>[6x]SVRDELRWVF;>MPKALRFLGWPVLVGVLLALLIIQHNPELVGLPRQEVHVEQAPLLSRLQEGPVSYANAVSRAAPAVANLYTTKMVSKPSHPLFDDPMFRRFFGDNLPQQKRMESSLGSAVIMSAEGYLLTNNHVTAGADQIIVALRDGRETIAQLVGSDPETDLAVLKIDLKNLPAMTLGRSDGIRTGDVCLAIGNPFGVGQTVTMGIISATGRNQLGLNTYEDFIQTDAAINPGNSGGALVDAAGNLIGINTAIFSKSGGSQGIGFAIPTKLALEVMQSIIEHGQVIRGWLGVEVKALTPELAESLGLGETAGIVVAGVYRDGPAARGGLLPGDVILTIDKQEASDGRRSMNQVARTRPGQKISIVVLRNGQKVNLTAEVGLRPPP[6x]

AlgW, a membrane-bound periplasmic serine protease belonging to the HtrA protein family, is a key regulator of the regulated intramembrane proteolysis (RIP) pathway and is responsible for transmitting the envelope stress signals in Pseudomonas aeruginosa. The AlgW PDZ domain senses and binds the C-terminal of mis-localized outer membrane proteins (OMPs) or periplasmic protein MucE, leading to catalytic activation of the protease domain. HtrA protease is characterized by its trypsin-like catalytic domain and regulatory PDZ domain; the catalytic triad was surrounded by several loops (L1, L2, L3, LD, LA) but, usually, in an inactive mode, and could be activated by sensing a specific molecular stimulus. The catalytic triad (H123, D153, and S227) sites are located between two β-barrels and are surrounded by activation loops L1 to L3, LD, and LA (named according to DegS nomenclature).

Protein samples were mixed with two types of peptide activator (tripeptide WVF, decapeptide SVRDELRWVF) prior to crystallization trials, yielding four complex structures, AlgW-tripeptide, AlgWS227A-tripeptide, AlgW-decapeptide, and AlgWS227A-decapeptide, with resolutions from 1.8 to 2.6 Å. In AlgW-decapeptide, each asymmetric unit contains a DegP-like hexamer that is stacked by two interlocked basic trimers arranged in a face-to-face manner, whereas the intertrimer contacts are stabilized by the long LA loop extending from the protease domain into the PDZ domain of another trimer. AlgWS227A-decapeptide could even generate a DegQ-like “cage” architecture after symmetry operation; the dodecamer of soluble AlgW contains four trimers, with the 12 LA loops protruding toward the interior of the cage. LA-mediated higher oligomerization is an important regulation mechanism in the HtrA family; however, very few close contacts are observed between trimers in AlgW-decapeptide and AlgWS227A-decapeptide structures, indicating that crystal packing may, in fact, dominate the above-described intertrimer associations. Fortunately, LA loops could be reliably modeled in AlgW-decapeptide and AlgWS227A-decapeptide structures, allowing us to explore the conformational regulation mode of the LA loop. By comparing the two sets of decapeptide-bound structures, we found that the LA loop shows joint angle shifts of about 7.65 degrees. In the AlgW-decapeptide structure, T72 forms side chain hydrogen interactions with D130 to maintain the β1-β4 association, while in β2, the side chain flipping of L106 not only disrupted T71-V124 interaction but also changed the dihedral angles of S105, leading β2 to form a long antiparallel sheet with β1. Additionally, K73 and E103 also altered their side chain orientations to adapt to the conformational changes. Eventually, these structural variations released the LA loop outward and exposed the active center.>[4x]QGRKYSYEAEKRSAVTLTNENFKSRKNKTTALSDQNHRFVPYFGSSEWLRFDALHPAVLAEKYDRNYRPYFIGQRGSASLNQYLGMQQMLPELQNGTAVYVLSPQWFTKKGYNSAAFQQFFNNDQLSSFLSQNQTDANSQYAAKRILEMKPEITMKSQLSKVAKGQDLNTVDKTYIQFMAELNRREDSLF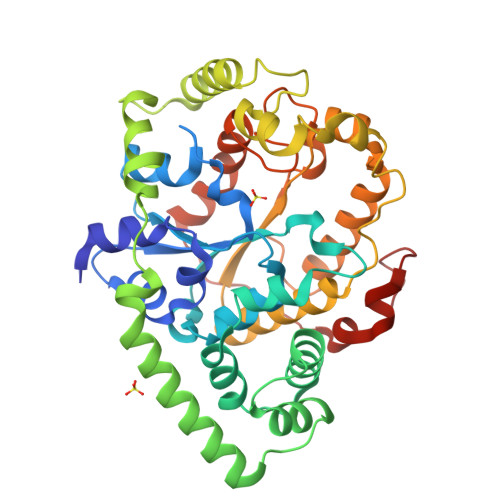SPLAASNNANYDKKVLPYLKELPDQFSYDALDQLAVRDAEAHTKSNDFGIDDRFYKERLSKKIGKLKGFQKNLSYEVSQEYGDLQLVLNQFAKSNTNVIFVIPPVNSKWMAYTGLNQDMYDATVSKIRYQLESQGFTNIADFSKDGDQPYFMQDTIHMGWKGWVAFDRVVNSFVSNPTPAPSYKLNDRFYSKDWSGYTGTPSQFKDE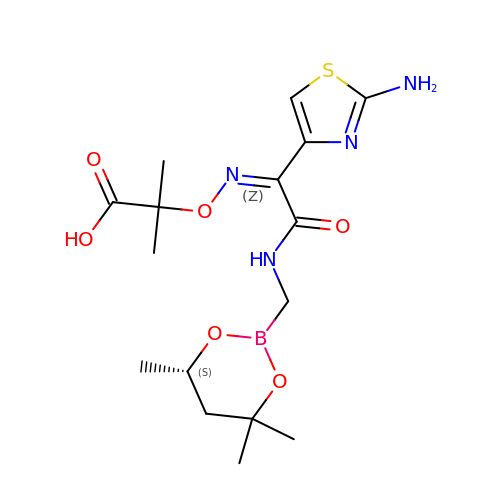2-[(~{Z})-[1-(2-azanyl-1,3-thiazol-4-yl)-2-oxidanylidene-2-[[(6~{S})-4,4,6-trimethyl-1,3,2-dioxaborinan-2-yl]methylamino]ethylidene]amino]oxy-2-methyl-propanoic acid | C16 H25 B N4 O6 S | VUZFEPQBACFWNR-GAGKSFBISA-N>[2x]MVDVVMAPCSPVECRTAVVIDVLRATSTIVTALSNGASGVIPVKTIEEALEKKKEGVLICGERNAQKPKGF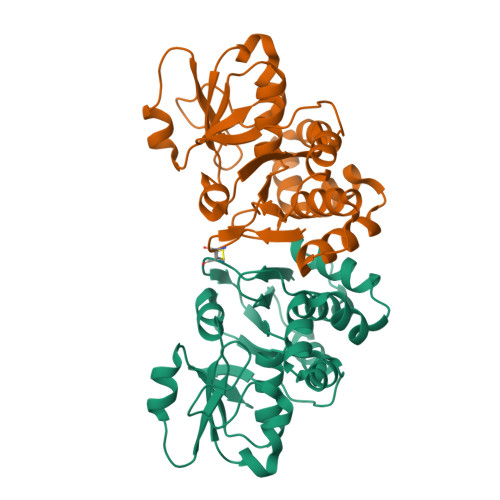NLGNSPLEYRKEKISGKTIVLTTTNGTQVIEKIRSEEIIAASFLNLSAVVEYLKSKEDILLVCAGTNGRFSLEDFLLAGAIVKRLKRNDLGDGAHAAERYFESVENTREEIKKHSSHAKRLISLGFENDIEFCTTEDLFKTVPALVNGVFILKEFP>MLEETEAALLARVRELFGATLRQVEPLTGTWTNEDVHRLFLAPPSVFLAWMGCGEGRTRREVESRWAFFVVAELLNGEPVNRPGIYQIVERLIAGVNGQTFGPTTGMRLTQVRNLCDDNRINAGVVLYGVLFSGTTPLPSVVDLDSLDDYERHWQTWKFPDETPEFAAHINVNQEKDHDAEN[6x];>MSDISFNAIPSDVRVPLTYIEFDNSNAVSGTPAPRQRVLMFGQSGSKASAAPNVPVRIRSGSQASAAFGQGSMLALMADAFLNANRVAELWCIPQGNGTGNAAVGEISLSGTAGENGSLVTYIAGQRLAVSVAAGATGAALADLLVARIKGQPDLPVTAEVRADSGDDDTHADVVLSAKFTGALSAVDVRWNYYAGETTPYGIITAFKAASGKNGNPDISASIAGMGDLQYKYIVMPYTDEPNLNLLRTELQERWGPVNQADGFAVTVLSGTYGDISTFGVSRNDHLISCMGIAGAPEPSYLYAATLCAVASQALSIDPARPLQTLTLPGRMPPAVGDRFTWSERNALLFDGISTFNVNDGGEMQIERMITMYRTNKYGDSDPSYLNVNTIATLSYLRYSLRTRITQKFPNYKLASDGTRFATGQAVVTPSVIKTELLALFEEWENAGLVEDFDTFKEELYVARNKDDKDRLDVLCGPNLINQFRIFAAQVQFIL[12x];>MAGNQRQGVAFIRVNGMELESMEGASFTPSGITREEVTGSRVYGWKGKPRAAKVECKIPGGGPIGLDEIIDWENITVEFQADTGET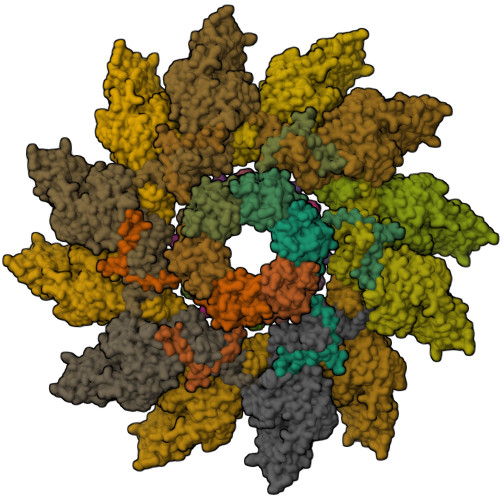WMLANAWQADEPKNDGGEISLVLMAKQSKRIA[12x]>MTSKSSAFRRLTAAVGTVAVAVAGVISMGQVASAQQATAVGPDQPGAPTHGSLTVHKYVGQEGNAGTGEEISVPGGQPLEGAEFTIWRLGTNDGDSCEPIDLANTNDWAQVPTGAAPRELSAVQNDFCLVDGGTARTTNSAGEYTFGNLDLGLYYVQETDAPANIVSRTAPFYVSIPLPHAQQNWLYDVHVYPKNQEVDAPTKTINSDSDQAGKGLTVGSVVEWTISQTVPALNDGEQYTSATIWDVLNPAELEYAGTTSVSLNGTPLVEGTDYTIDAGVVSWSLTEKKLAEIKAGDTIEVVFTTTVLAVTETGDIDNPGSEGPDKPGYGSEFNGGTTPGGTTPHTYWGQLTVNKGDTGMVNKLAGAEFAVFNNAENGVCAPEAPETDAIATGVSDAEGVVRWNDVTPDNPLGLWIANSSDGEIANPNKDYCLYETKAPSGYVAGPVQKVNITPGTTAKLVV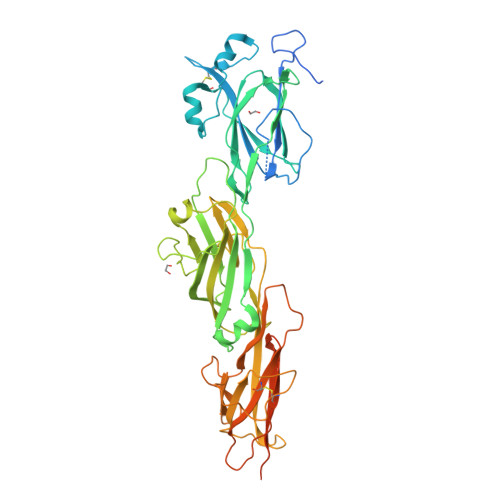DFENTKKDGPNLPLTGGQGTLMMTIGGLALMLVGAGAVYALRRRNEA[2x]> MRDRQAFERAKDLQAVIFDKTGTLTEGRFGVTDIVGFNHSEDELLQIAASLEARSEHPIAAAIVEEAEKRGFGLTEVEEFRAIPGKGVEGIVNGRRYMVVSPGYIRELGIKTDESVEKLKQQGKTVVFILKNGEVSGVIALADRIRPESREAISKLKAIGIKCMMLTGDNRFVAKWVAEELGLDDYFAEVLPHEKAEKVKEVQQKYVTAMVGDGVNDAPALAQADVG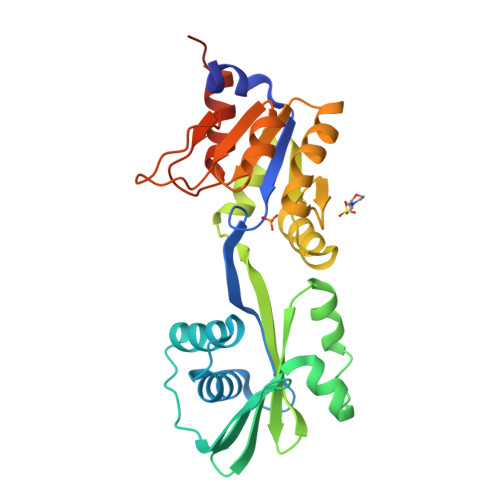IAIGAGTDVAVETADIVLVRNDPRDVAAIVELSRKTYSKLEHHHHHH Here, we describe the crystal structures of the N-terminal RD and the C-terminal ED of the lantibiotic resistance-associated RR NsrR from S. agalactiae. NsrR is part of the nisin resistance operon. The expression of the genes of this operon is induced by a TCS consisting of the HK NsrK and the RR NsrR. NsrR belongs to the OmpR/PhoB family of RRs.

The structure of the NsrR-RD was determined at a resolution of 1.8 Å. The asymmetric unit contains two copies of NsrR-RD. NsrR-RD structurally adopts a αβ doubly-wound fold previously observed in OmpR/PhoB type regulators. Five β-strands (β1-β5) are arranged in a parallel fashion constituting the central core of the structure, which is surrounded by two α-helices (α1 and α5) on one and three helices (α2, α3, α4) on the other side. Superimposition of the structures revealed that helix α4 is slightly rotated outward in NsrR-RD. Furthermore, helix α4 in NsrR is shorter than in other RRs. The putative phosphorylation site of NsrR is Asp55, which is localized at the end of strand β3 and lies within an acidic environment composed of the side chains of Glu12 and Asp13 (highlighted in pink). However, the structure of NsrR-RD did not contain any divalent ion. Instead, a water molecule is present, which interacts with Glu12 of the acidic pocket, Lys104, and another water molecule in the vicinity.

>[2x]MSQEQGKIYIVEDDMTIVSLLKDHLSASYHVSSVSNFRDVKQEIIAFQPDLILMDITLPYFNGFYWTAELRKFLTIPIIFISSSNDEMDMVMALNMGGDDFISKPFSLAVLDAKLTAILRRSQQFIQQELTFGGFTLTREGLLSSQDKEVILSPTENKILSILLMHPKQVVSKESLLEKLWENDSFIDQNTLNVNMTRLRKKIVPIGFDYIHTVRGVGYLLQDPNSSSVDKLAAALEHHHHHH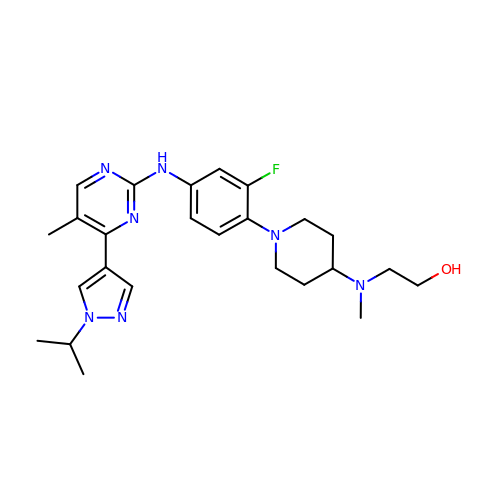2-((1-(2-fluoro-4-((4-(1-isopropyl-1H-pyrazol-4-yl)-5-methylpyrimidin-2-yl)amino)phenyl)piperidin-4-yl)(methyl)amino)ethan-1-ol | C25 H34 F N7 O | CVLXNRIQVFIVGY-UHFFFAOYSA-N> SSLRLPSAAELSGQWVLSGAEQHCDIRLNTDVLDGTTWKLAGDTACLQKLLPEAPVGWRPTPDGLTLTQADGSAVAFFSRNRDRYEHKLV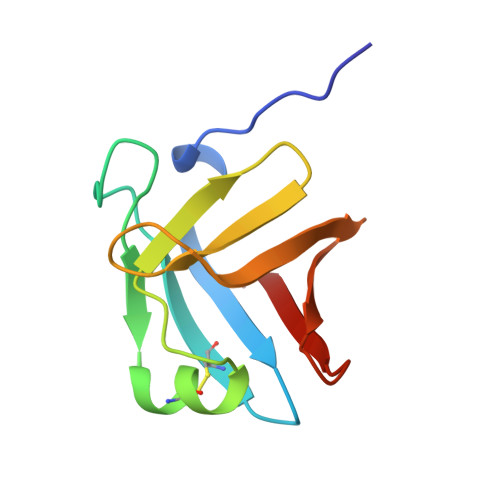DGSVRTLKKKA GUANOSINE-5',3'-TETRAPHOSPHATE 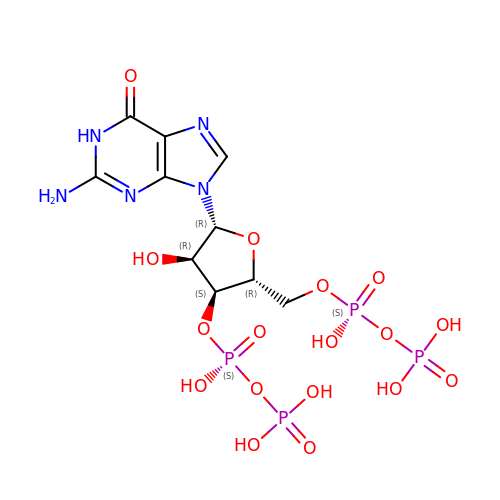| C10 H17 N5 O17 P4 | BUFLLCUFNHESEH-UUOKFMHZSA-N>[2x]ACTCGG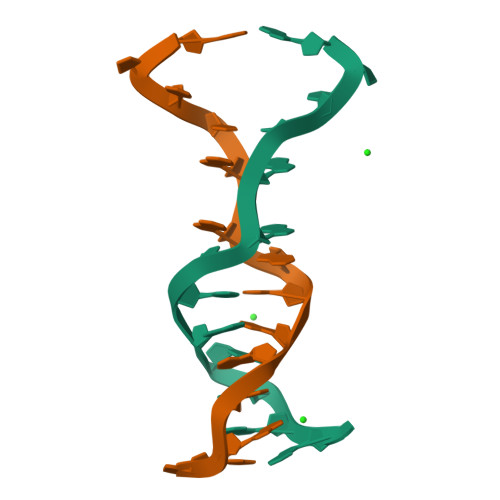ACGACGAT>[2x]MGLEQLEAQTNFTKRELQVLYRGFKNECPSGVVNEDTFKQIYAQFFPHGDASTYAHYLFNAFDTTQTGSVKFEDFVTALSILLRGTVHEKLRWTFNLYDINKDGYINKEEMMDIVKAIYDMMGKYTYPVLKEDTPRQHVDVFFQKMDKNKDGIVTLDEFLESCQEDDNIMRSLQLFQNVM;>[2x]AAWLPFARAAAIGWMPVANCPMPL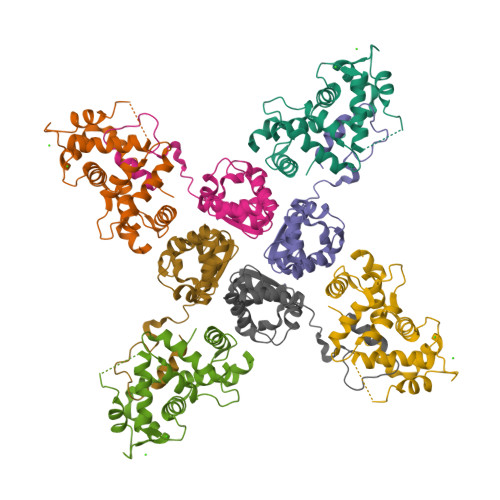APADKNKRQDELIVLNVSGRRFQTWRTTLERYPDTLLGSTEKEFFFNEDTKEYFFDRDPEVFRCVLNFYRTGKLHYPRYECISAYDDELAFYGILPEIIGDCCYEEYKDRKRENAE> MASSRCPAPRGCRCLPGASLAWLGTVLLLLADWVLLRTALPRIFSLLVPTALPLLRVWAVGLSRWAVLWLGACGVLRATVGSKSENAGAQGWLAALKPLAAALGLALPGLALFRELISWGAPGSADSTRLLHWGSHPTAFVVSYAAALPAAALWHKLGSLWVPGGQGGSGNPVRRLLGCLGSETRRLSLFLVLVVLSSLGEMAIPFFTGRLTDWILQDGSADTFTRNLTLMSILTIASAVLEFVGDGIYNNTMGHVHSHLQGEVFGAVLRQETEFFQQNQTGNIMSRVTEDTSTLSDSLSENLSLFLWYLVRGLCLLGIMLWGSVSLTMVTLITLPLLFLLPKKVGKWYQLLEVQVRESLAKSSQVAIEALSAMPTVRSFANEEGEAQKFREKLQEIKTLNQKEAVAYAVNSWTTSISGMLLKVGILYIGGQLVTSGAVSSGNLVTFVLYQMQFTQAVEVLLSIYPRVQKAVGSSEKIFEYLDRTPRCPPSGLLTPLHLEGLVQFQDVSFAYPNRPDVLVLQGLTFTLRPGEVTALVGPNGSGKSTVAALLQNLYQPTGGQLLLDGKPLPQYEHRYLHRQVAAVGQEPQVFGRSLQENIAYGLTQKPTMEEITAAAVKSGAHSFISGLPQGYDTEVDEAGSQLSGGQRQAVALARALIRKPCVLILDDATSALDANSQLQVEQLLYESPERYSRSVLLITQHLSLVEQADHILFLEGGAIREGGTHQQLMEKKGCYWAMVQAPADAPE;> MRLPDLRPWTSLLLVDAALLWLLQGPLGTLLPQGLPGLWLEGTLRLGGLWGLLKLRGLLGFVGTLLLPLCLATPLTVSLRALVAGASRAPPARVASAPWSWLLVGYGAAGLSWSLWAVLSPPGAQEKEQDQVNNKVLMWRLLKLSRPDLPLLVAAFFFLVLAVLGETLIPHYSGRVIDILGGDFDPHAFASAIFFMCLFSFGSSLSAGCRGGCFTYTMSRINLRIREQLFSSLLRQDLGFFQETKTGELNSRLSSDTTLMSNWLPLNANVLLRSLVKVVGLYGFMLSISPRLTLLSLLHMPFTIAAEKVYNTRHQEVLREIQDAVARAGQVVREAVGGLQTVRSFGAEEHEVCRYKEALEQCRQLYWRRDLERALYLLVRRVLHLGVQMLMLSCGLQQMQDGELTQGSLLSFMIYQESVGSYVQTLVYIYGDMLSNVGAAEKVFSYMDRQPNLPSPGTLAPTTLQGVVK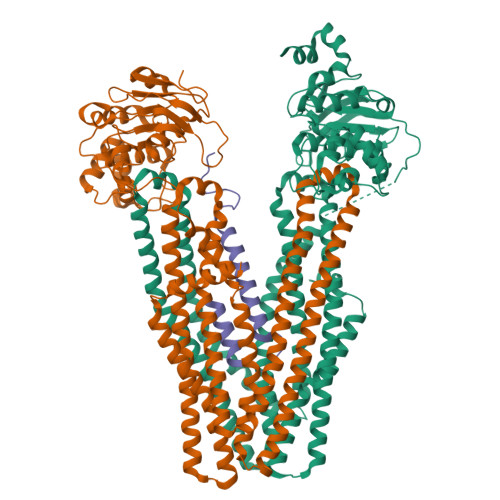FQDVSFAYPNRPDRPVLKGLTFTLRPGEVTALVGPNGSGKSTVAALLQNLYQPTGGQVLLDEKPISQYEHCYLHSQVVSVGQEPVLFSGSVRNNIAYGLQSCEDDKVMAAAQAAHADDFIQEMEHGIYTDVGEKGSQLAAGQKQRLAIARALVRDPRVLILDEATSALDVQCEQALQDWNSRGDRTVLVIAHRLQTVQRAHQILVLQEGKLQKLAQL;> MSWALEMADTFLDNMRVGPRTYADVRDEINKRGREDREAARTAVHDPERPLLRSPGLLPEIAPNASLGVVHRRTGGTVTDSPRNPVTR> ANIVGGIEYSINNAS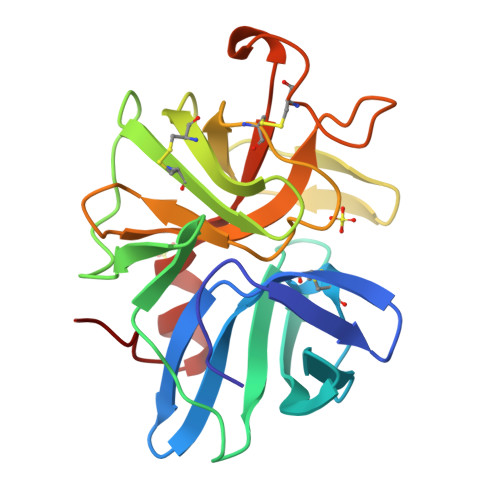LCSVGFSVTRGATKGFVTAGHCGTVNATARIGGAVVGTFAARVFPGNDRAWVSLTSAQTLLPRVANGSSFVTVRGSTEAAVGAAVCRSGRTTGYQCGTITAKNVTANYAEGAVRGLTQGNACAGRGDSGGSWITSAGQAQGVMSGLNVQSNGNNCGIPASQRSSLFERLQPILSQYGLSLVTG>[2x]MSRKSRNCRNPPRSGDAQQRPRERSGSGMSTTPLQVLPGAE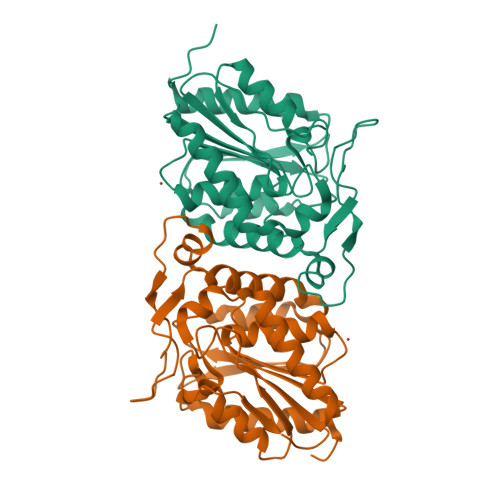PLYSVGSRIGVLVSHGFTGSPQSMRFLAEGFARAGYTVATPRLTGHGTTPAEMAASTASDWTADIVAAMRWLEERCDVLFMTGLSMGGALTVWAAGQFPERFAGIMPINAALRMESPDLAALAFNPDAPAELPGIGSDIKAEGVKELAYPVTPVPAIKHLITIGAVAEMLLPRVKCPALIIQSREDHVVPPHNGELIYNGIGSTEKELLWLENSYHVATLDNDKELILERSLAFIRKHSKLAAALEHHHHHH> MMRHTVVRHHRTGKARAFIMRDPSLKILRAGSGFQQLKRMGMPSQKTLGYRQVDNFYANNQYQHAWPLLTHDDLGNSDQSNQTKNILYSMYMPKRNKGTAPWFRGADTYSVKYCEQGRYEYQRYLMINRFPSEYKRHFLRFLGNIRGSKSRDAVPQEALHWLLRMIVDNFNPQHVHYIAAMRTLQDSGELDMARDVWKIMERQQTWPDTATICAYLDVCVEAGEKTWAVEAWNRYCTELRFLQAGEVDPKPITRTPFSLTREELLYLPKWKKHFDHDPNLDVPDLNRFNRTREVYLRMAKVMLASDDMSMFEHFFDKLQAAMLTTPTPVPEPPNPHLVRRPRWSPYEHQKSLHHSPWRMDNNGRAMALGPSRTIEGEMQSRFFSNPQFLVHAVKEAVAVVLQRHMAMFPEATDAQTAAPAFFELTETAQETLAFCDGLVQRMMERLEDKLGSLGTSSLLSTLLCIRRVVGKQSGRALLEYANQFLAKKATLSADGLRESLTAPNYFQILAAYADESAYHYDPKTRQYTYAPGFRPTETMKGLSATLNEISANQHVAWSAEMHLQVVRTLVGCGTMKANAYFVENVLRQFKWDSRFLEALYAEYRRHNTVDGWAELTKRALVWTARYNVIASERLKRLIEDDYDIIHVQTRTFRELAVFQFRDAEEKRHARDVVNELPNPWIDYVTHALPFPDRDAGYPDEYGDIGQWRAPGGPGSPVKGPGYYAPPMEGEHMRGYTAEWRDLKNPMKPPAFPEPWERKYKQYARGQHPSYDMVYAGPMPEIF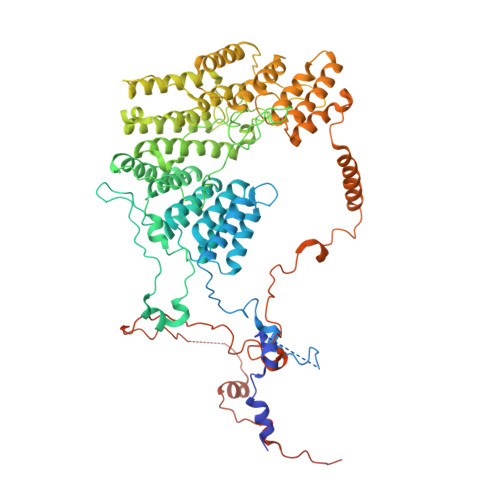PGRRDFRKPTRWDYHDVEKQGKHKISGPY>GPMAKKRTYQGKVPLHDNYGPEAKYAVEAEALLPTTKFEEEIARGLELGLPGADSIKDRRIPTFSRGELPHFAGINTFIKAPYVEDVRKCGQYDVAILGAPFDGGTTYRAGTRFGPQGIRKISALYGTYSFELGVDLRESVSICDVGDIFTIPGNIEKTFDQVSKGVGHVFASGAFPVVLGGDHSLGFATVRGVAQHLNGKKLGILHFDRHVDTQDTDLDERMHTTPWFHATNIPNVPAKNLVQIGIGGWQAPRPGVKAGRERQTTIMTVTDCVEMGIENAAKQALEVAFDGVDAVWLSFDVDCLDAAFVPGTGWPEPGGFLPREVLKFLQIIADTKPLAGMEIVECAPPYDAAEITSLMATRVICDVLACQVRSGHLGNRKKR[12x]

Proteomics, enzyme kinetics and the crystal structure of a N. inopinata guanidinase homologue demonstrated that it is a bona fide guanidinase. Phylogenetic analyses revealed that the comammox guanidinases belong to the ureohydrolase enzyme superfamily. Substrates converted by this enzyme family typically contain a guanidine moiety, which is hydrolysed to release urea. In 2021, a Ni-containing guanidinase, mediating the direct hydrolysis of free guanidine to urea (which is further converted by urease to ammonia and CO2) and ammonia, was described in a Synechocystis strain.

The guanidinase enzyme of N. inopinata was expressed in E. coli, purified to homogeneity and characterized as a homohexamer with a molecular mass of 240 kDa, resembling the recently discovered guanidinase of Synechocystis sp. PCC6803 (GdmH). Crystal structure analyses of the heterologously expressed N. inopinata guanidinase (resolution of 1.58 Å) revealed that it exhibits the same α-β-α fold of the arginase subfamily as its cyanobacterial homologue, but with each subunit containing one nickel and one manganese ion with the overall structure being highly similar to the Synechocystis enzyme with an root mean squared deviation of 0.74 Å over an aligned length of 361 Cα atoms. However, the N. inopinata guanidinase possesses an N-terminal extension, which is lacking in the cyanobacterial enzyme. This extension stabilizes the tertiary and quaternary structure of the guanidinase through extensive interactions, consistent with its notably high thermostability and activity in a wide pH range. On the other hand, in comparison to the cyanobacterial enzyme, the N. inopinata guanidinase lacks a C-terminal extension. In the active site of the heterologously expressed N. inopinata guanidinase, one nickel and one manganese ion are coordinated through conserved histidine and aspartic acid residues. The positions and identity of metal sites were determined by the diffraction anomalous dispersion signal and corroborated by inductively coupled plasma mass spectrometry (ICP-MS) metal analysis. Another notable difference between the active sites of the Synechocystis and the N. inopinata enzymes is a tilt of N. inopinata guanidinase Trp313 towards the active-site nickel ion. The tilted Trp313 in N. inopinata guanidinase permits access to the active site from the surface, in contrast to Trp305 of the cyanobacterial enzyme, which blocks it. The hexamer’s ridges display a negative electrostatic potential, and each cavity marks the start of a 17 Å negatively charged tunnel towards the active site.> GSHMSNTQTVLPFTGLNTPSGVAVDSAGTVYVTDHGNNRVVKLAAGSNTQTVLPFTGLNTPHGVAVDSAGTVYVTDHGNNRVVKLAAGSNTQTVLPFTGLNTPSGVAVDSAGT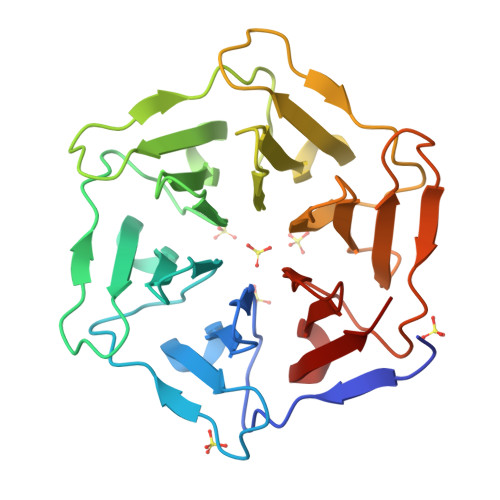VYVTDHGNNRVVKLAAGSNTQTVLPFTGLNTPHGVAVDSAGTVYVTDHGNNRVVKLAAGSNTQTVLPFTGLNTPSGVAVDSAGTVYVTDHGNNRVVKLAAGSNTQTVLPFTGLNTPHGVAVDSAGTVYVTDHGNNRVVKLAAG2-[(1R)-1-CARBOXY-2-(4-HYDROXYPHENYL)ETHYL]-1,3-DIOXOISOINDOLINE-5-CARBOXYLIC 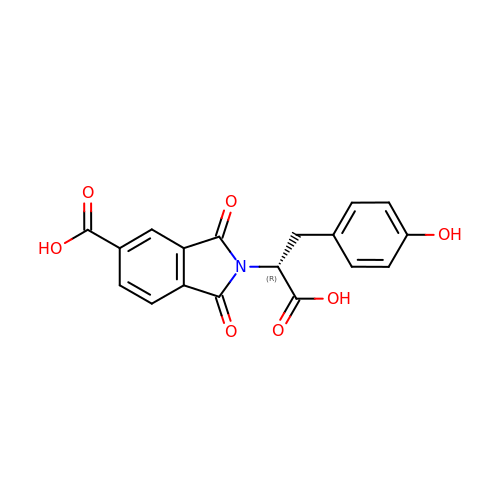ACID | C18 H13 N O7 | QISJEFYTLZTWIQ-CQSZACIVSA-N>[4x]MWSHPQFEKIEGRMQNDILQVVSQGWKYFKGNFYYFSLIPKTWYSAEQFCVSRNSHLTSVTSESEQEL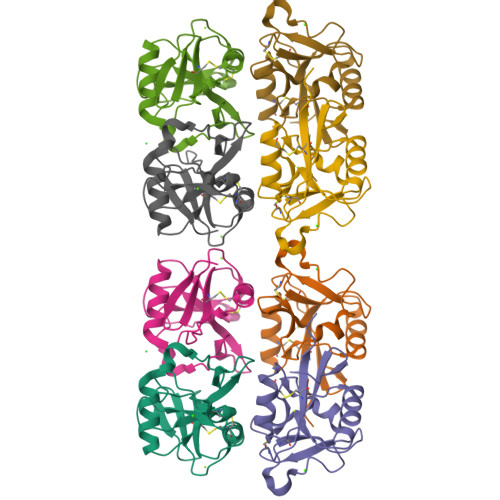LYKTAGGLIYWIGLTKAGMEGDWSWVDDTPFNKVQSARFWIPGEPNNAGNNEHCGNIKAPSLQAWNDAPCDKTFLFICKRPYVPSEP> GSHMGSPNSPLKDSLRPKLSEEQQHIIAILLDAHHKTYDPTYADFRDFRPPVRMDGSTGSVTLDLSPLSMLPHLADLVSYSIQKVIGFAKMIPGFRDLTSDDQIVLLKSSAIEVIMLRSNQS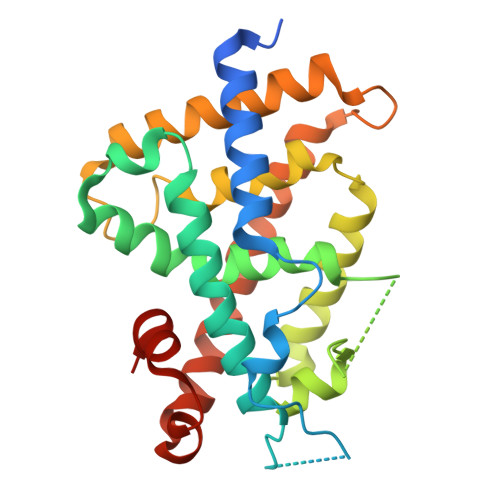FTMDDMSRDCGSQDYKYDVTDVSKAGHTLELIEPLIKFQVGLKKLNLHEEEHVLLMAICIVSPDRPGVQDAKLVEAIQDRLSNTLQTYIRCRHPPPGSHQLYAKMIQKLADLRSLNEEHSKQYRSLSFQPENSMKLTPLVLEVFGNEIS> GAMAKGAVTKLKFNSP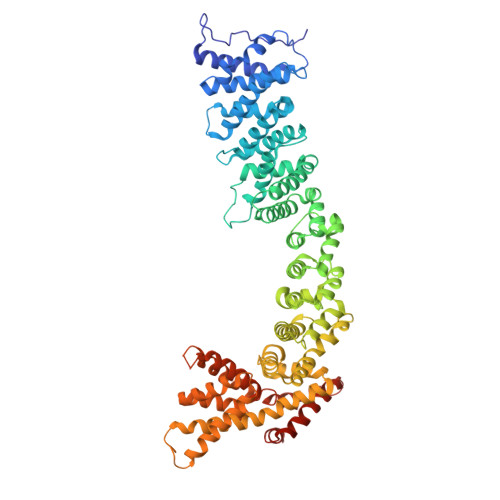IISTSDQLISTNELLDRLKALHEELASLDQDNTDLTGLDKYRDALVSRKLLKHKDVGIRAFTACCLSDILRLYAPDAPYTDAQLTDIFKLVLSQFEQLGDQENGYHIQQTYLITKLLEYRSIVLLADLPSSNNLLIELFHIFYDPNKSFPARLFNVIGGILGEVISEFDSVPLEVLRLIFNKFLTYNPNEIPEGLNVTSDCGYEVSLILCDTYSNRMSRHLTKYYSEIIHEATNDDNNSRLLTVVVKLHKLVLRLWETVPELINAVIGFIYHELSSENELFRKEATKLIGQILTSYSDLNFVSTHSDTFKAWISKIADISPDVRVEWTESIPQIIATREDISKELNQALAKTFIDSDPRVRRTSVMIFNKVPVTEIWKNITNKAIYTSLLHLAREKHKEVRELCINTMAKFYSNSLNEIERTYQNKEIWEIIDTIPSTLYNLYYINDLNINEQVDSVIFEYLLPFEPDNDKRVHRLLTVLSHFDKKAFTSFFAFNARQIKISFAISKYIDFSKFLNNQESMSSSQGPIVMNKYNQTLQWLASGLSDSTKAIDALETIKQFNDERIFYLLNACVTNDIPFLTFKNCYNELVSKLQTPGLFKKYNISTGASIMPRDIAKVIQILLFRASPIIYNVSNISVLLNLSNNSDAKQLDLKRRILDDISKVNPTLFKDQIRTLKTIIKDLDDPD> GSTPPPFPGEPWKVSVNVHSFKPEELMVKTKDGYVEVSGKHEEKQQEGGIVSKNFTKKIQLPAEVDPVTVTSSLSPEGL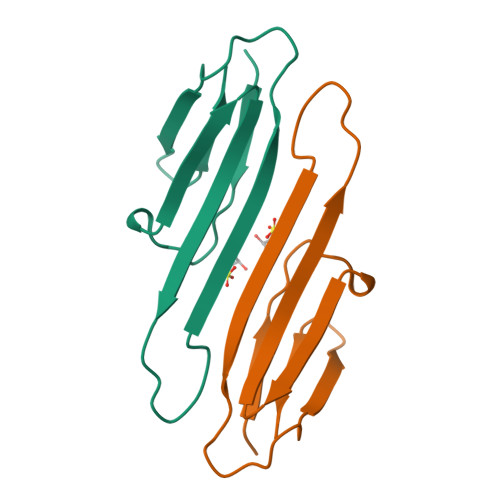LIIEA> MFGLPQ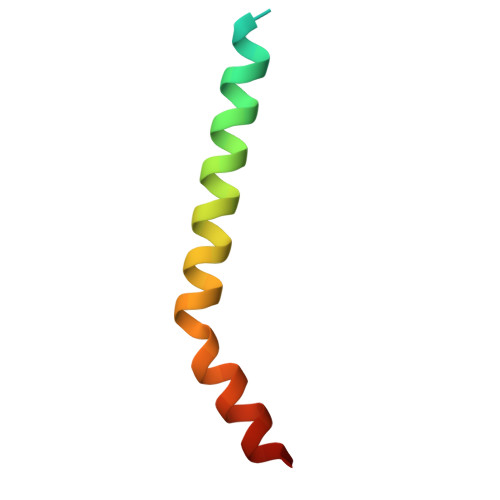QEVSEEEKRAHQEQTEKTLKQAAYVAAFLWVSPMIWHLVKKQWK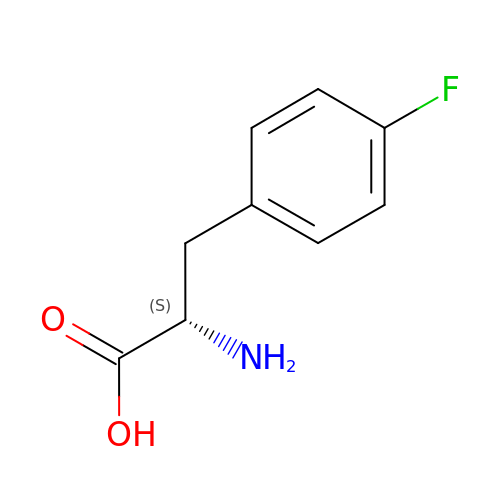4-FLUORO-L-PHENYLALANINE | C9 H10 F N O2 | XWHHYOYVRVGJJY-QMMMGPOBSA-N>GSMASLPVLQKESVFQSGAHAYRIPALLYLPGQQSLLAFAEQRASKKDEHAELIVLRRGDYDAPTHQVQWQAQEVVAQARLDGHRSMNPCPLYDAQTGTLFLFFIAIPGQVTEQQQLETRANVTRLCQVTSTDHGRTWSSPRDLTDAAIGPAYREWSTFAVGPGHCLQLNDRARSLVVPAYAYRKLHPIQRPIPSAFCFLSHDHGRTWARGHFVAQDTLECQVAEVETGEQRVVTLNARSHLRARVQAQSTNDGLDF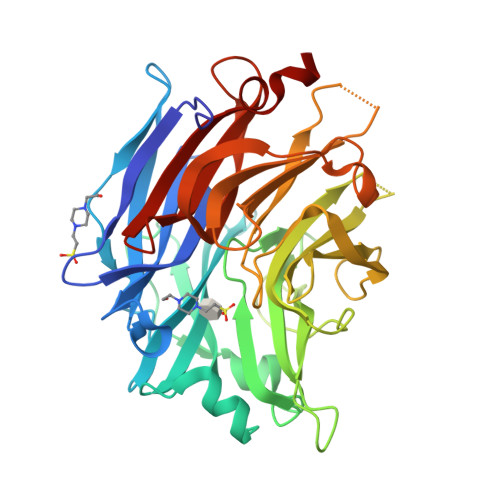QESQLVKKLVEPPPQGCQGSVISFPSPRSGPGSPAQWLLYTHPTHSWQRADLGAYLNPRPPAPEAWSEPVLLAKGSCAYSDLQSMGTGPDGSPLFGCLYEANDYEEIVFLMFTLKQAFPAEYLPQ[2x]> SGISLDNSYKMDYPEMGLCIIINNKNFHKSTGMTSRSGTDVDAANLRE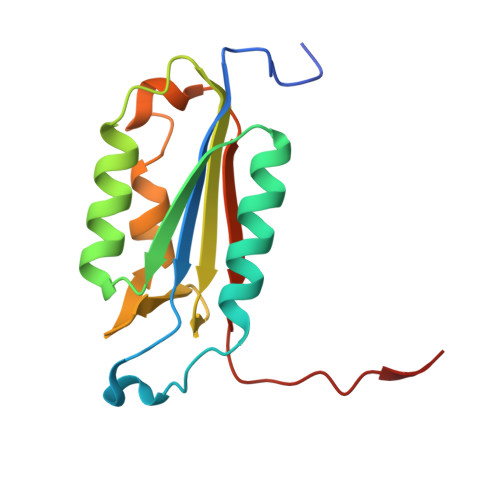TFRNLKYEVRNKNDLTREEIVELMRDVSKEDHSKRSSFVCVLLSHGEEGIIFGTNGPVDLKKITNFFRGDRCRSLTGKPKLFIIQACRGTEDDCGIETD> KDIEISASESKFILEALRQNYRLDGRSFDQFRDVEITFGKEFGDVSVKMGNTKVHCRISCQIAQPYEDRPFEGLFVISTEISPMAGSQFENGNITGEDEVLCSRIIEKSVRRSGALDVEGLCIVAGSKCWAVRADVHFLDCDGGFIDASCIAVMAGLMHFKKPDITVHGEQIIVHPVNEREPVP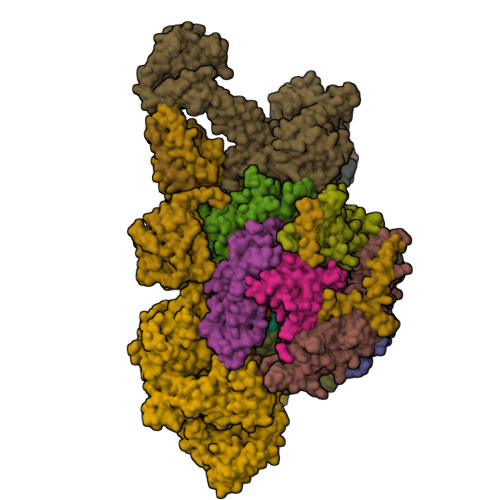LGILHIPICVTFSFFNPQDTEENIKGETNSEISIIDATLKEELLRDGVLTVTLNKNREVVQVSKAGGLPMDALTLMKCCHEAYSIIEKITDQILQLLKEDSEKRNKYAAMLTSENAREI;> GHMSRLEIYSPEGLRLDGRRWNELRRFESSINTHPHAADGSSYMEQGNNKIITLVKGPKEPRLKSQMDTSKALLNVSVNITKFSKFERSKSSHKNERRVLEIQTSLVRMFEKNVMLNIYPRTVIDIEIHVLEQDGGIMGSLINGITLALIDAGISMFDYISGISVGLYDTTPLLDTNSLEENAMSTVTLGVVGKSEKLSLLLVEDKIPLDRLENVLAIGIAGAHRVRDLMDEELRKHAQKRVSNASAR;> AESTTLETIEIHPITFPPEVLARISPELSLQRHLSLGIRPCLRKYEEFRDVAIENNTLSRYADAGNIDTKNNILGSNVLKSGKTIVITSITGGIIEETSASIKDLDDFGEEELFEVTKEEDIIANYASVYPVVEVERGRVGACTDEEMTISQKLHDSILHSRILPKKALKVKAGVRSANEDGTFSVLYPDELEDDTLNETNLKMKRKWSYVLYAKIVVLSRTGPVFDLCWNSLMYALQSVKLPRAFIDERASDLRMTIRTRGRSATIRETYEIICDQTKSVPLMINAKNIAFASNYGIVELDPECQLQNSDNSEEEEVDIDMDKLNTVLIADLDTEAEETSIHSTISILAAPSGNYKQLTLMGGGAKITPEMIKRSLLLSRVRADDLSTRFNI;> GHGNNKEPNTKNRLDSAEKKKKMSVQAEIGILDHVDGSSEFVSQDTKVICSVTGPIEPKARQELPTQLALEIIVRPAKGVATTREKVLEDKLRAVLTPLITRHCYPRQLCQITCQILESGEDEAEFSLRELSCCINAAFLALVDAGIALNSMCASIPIAIIKDTSDIIVDPTAEQLKISLSVHTLALEFVNGGKVVKNVLLLDSNGDFNEDQLFSLLELGEQKCQELVTNIRRIIQDNISPRLVV;> GHMSLSVAEKSYLYDSLASTPSIRPDGRLPHQFRPIEIFTDFLPSSNGSSRIIASDGSECIVSIKSKVVDHHVENELLQVDVDIAGQRDDALVVETITSLLNKVLKSGSGVDSSKLQLTKKYSFKIFVDVLVISSHSHPISLISFAIYSALNSTYLPKLISAFDDLEVEELPTFHDYDMVKLDINPPLVFILAVVGNNMLLDPAANESEVANNGLIISWSNGKITSPIRSVALNDSNVKSFKPHLLKQGLAMVEKYAPDVVRSLENL;> MNVQDRRRLLGPAAAKPMAFSNTTTHVPEKKSTDLTPKGNESEQELSLHTGFIENCNGSALVEARSLGHQTSLISAVYGPRSIRGSFTSQGTISIQLKNGLLEKYNTNELKEVSSFLMGIFNSVVNLSRYPKSGIDIFVYLTYDKDLTNNPQDDDSQSKMTSSQISSLIPHCITSITLALADAGIELVDMAGAGEANGTVVSFIKNGEEIVGFWKDDGDDEDLLECLDRCKEQYNRYRDLMISCLMNQET;> GHMSTFIFPGDSFPVDPTTPVKLGPGIYCDPNTQEIRPVNTGVLHVSAKGKSGVQTAYIDYSSKRYIPSVNDFVIGVIIGTFSDSYKVSLQNFSSSVSLSYMAFPNASKKNRPTLQVGDLVYARVCTAEKELEAEIECFDSTTGRDAGFGILEDGMIIDVNLNFARQLLFNNDFPLLKVLAAHTKFEVAIGLNGKIWVKCEELSNTLACYRTIMECCQKNDTAAFKDIAKRQFKEILTVKEE;> RSMSEVITITKRNGAFQNSSNLSYNNTGISDDENDEEDIYMHDVNSASKSESDSQIVTPGELVTDDPIWMRGHGTYFLDNMTYSSVAGTVSRVNRLLSVIPLKGRYAPETGDHVVGRIAEVGNKRWKVDIGGKQHAVLMLGSVNLPGGILRRKSESDELQMRSFLKEGDLLNAEVQSLFQDGSASLHTRSLKYGKLRNGMFCQVPSSLIVRAKNHTHNLPGNITVVLGVNGYIWLRKTSQMDLARDTPSANNSSSIKSTGPTGAVSLNPSITRLEEESSWQIYSDENDPSISNNIRQAICRYANVIKALAFCEIGITQQRIVSAYEASMVYSNVGELIEKNVMESIGSDILTAEKMRGNGN;> MKHHHHHHPMACNFQFPEIAYPGKLICPQYGTENKDGEDIIFNYVPGPGTKLIQYEHNGRTLEAITATLVGTVRCEEEKKTDQEEEREGTDQSTEEEKSVDASPNDVTRRTVKNILVSVLPGTEKGRKTNKYANNDFANNLPKEGDIVLTRVTRLSLQRANVEILAVEDKPSPIDSGIGSNGSGIVAAGGGSGAATFSVSQASSDLGETFRGIIRSQDVRSTDRDRVKVIECFKPGDIVRAQVLSLGDGTNYYLTTARNDLGVVFARAANGAGGLMYATDWQMMTSPVTGATEKRKCAKPF;> GAMSVPAIAPRRKRLADGLSVTQKVFVRSRNGGATKIVREHYLRSDIPCLSRSCTKCPQIVVPDAQNELPKFILSDSPLELSAPIGKHYVVLDTNVVLQAIDLLENPNCFFDVIVPQIVLDEVRNKSYPVYTRLRTLCRDSDDHKRFIVFHNEFSEHTFVERLPNETINDRNNRAIRKTCQWYSEHLKPYDINVVLVTNDRLNREAATKEVESNIITKSLVQYIELLPNADDIRDSIPQMDSFDKDLERDTFSDFTFPEYYSTARVMGGLKNGVLYQGNIQISEYNFLEGSVSLPRFSKPVLIVGQKNLNRAFNGDQVIVELLPQSEWKAPSSIVLDSEHFDVNDNPDIEAGDDDDNNESSSNTTVISDKQRRLLAKDAMIAQRSKKIQPTAKVVYIQRRSWRQYVGQLAPSSVDPQSSSTQNVFVILMDKCLPKVRIRTRRAAELLDKRIVISIDSWPTTHKYPLGHFVRDLGTIESAQAETEALLLEHDVEYRPFSKKVLECLPAEGHDWKAPTKLDDPEAVSKDPLLTKRKDLRDKLICSIDPPGCVDINDALHAKKLPNGNWEVGVHIADVTHFVKPGTALDAEGAARGTSVYLVDKRIDMLPMLLGTDLCSLKPYVDRFAFSVIWELDDSANIVNVNFMKSVIRSREAFSYEQAQLRIDDKTQNDELTMGMRALLKLSVKLKQKRLEAGALNLASPEVKVHMDSETSDPNEVEIKKLLATNSLVEEFMLLANISVARKIYDAFPQTAMLRRHAAPPSTNFEILNEMLNTRKNMSISLESSKALADSLDRCVDPEDPYFNTLVRIMSTRCMMAAQYFYSGAYSYPDFRHYGLAVDIYTHFTSPIRRYCDVVAHRQLAGAIGYEPLSLTHRDKNKMDMICRNINRKHRNAQFAGRASIEYYVGQVMRNNESTETGYVIKVFNNGIVVLVPKFGVEGLIRLDNLTEDPNSAAFDEVEYKLTFVPTNSDKPRDVYVFDKVEVQVRSVMDPITSKRKAELLLK;> MTSENPDVLLSRVINVVRAASSLASQDVDFYKNLDRGFSKDLKSKADKLADMANEIILSIDEHHESFELKEEDISDLWNNFGNIMDNLLEMSDHSLDKLNCAINSKSRGSDLQYLGEFSGKNFSPTKRVEKPQLKFKSPIDNSESHPFIPLLKEKPNALKPLSESLRLVDDDENNPSHYPHPYEYEIDHQEYSPEILQIREEIPSKSWDDSVPIWVDTSTELESMLEDLKNTKEIAVDLEHHDYRSYYGIVCLMQISTRERDYLVDTLKLRENLHILNEVFTNPSIVKVFHGAFMNIIWLQRDLGLYVVGLFDTYHASKAIGLPRHSLAYLLENFANFKTSKKYQLADWRIRPLSKPMTAYARADTHFLLNIYDQLRNKLIESNKLAGVLYESRNVAKRRFEYSKYRPLTPSSEVYSPIEKESPWKILMYQYNIPPEREVLVRELYQWRDLIARRDDESPRFVMPNQLLAALVAYTPTDVIGVVSLTNGVTEHVRQNAKLLANLIRDALRNIKNTNEEATPIPSSETKADGILLETISVPQIRDVMERFSVLCNSNISKSRAKPVTNSSILLGKILPREEHDIAYSKDGLPNKVKTEDIRIRAQNFKSALANLEDIIFEIEKPLVVPVKLEEIKTVDPASAPNHSPEIDNLDDLVVLKKKNIQKKQPAKEKGVTEKDAVDYSKIPNILSNKPGQNNRQQKKRRFDPSSSDSNGPRAAKKRRPAAKGKNLSFKR;> MEDIEKIKPYVRSFSKALDELKPEIEKLTSKSLDEQLLLLSDERAKLELINRYAYVLSSLMFANMKVLGVKDMSPILGELKRVKSYMDKAKQYDNRITKSNEKSQAEQEKAKNIISNVLDGNKNQFEPSISRSNFQGKHTKFENDELAESTTTKIIDSTDHIRKASSKKSKRLDKVGKKKGGKK;> MDSTDLFDVFEETPVELPTDSNGEKNADTNVGDTPDHTQDKKHGLEEEKEEHEENNSENKKIKSNKSKTEDKNKKVVVPMLADSFEQEASREVDASKGLTNSETLQVEQDGKVRLSHQVRHQVALPPNYDYTPIAEHKRVNEARTYPFTLDPFQDTAISCIDRGESVLVSAHTSAGKTVVAEYAIAQSLKNKQRVIYTSPIKALSNQKYRELLAEFGDVGLMTGDITINPDAGCLVMTTEILRSMLYRGSEVMREVAWVIFDEVHYMRDKERGVVWEETIILLPDKVRYVFLSATIPNAMEFAEWICKIHSQPCHIVYTNFRPTPLQHYLFPAHGDGIYLVVDEKSTFREENFQKAMASISNQIGDDPNSTDSRGKKGQTYKGGSAKGDAKGDIYKIVKMIWKKKYNPVIVFSFSKRDCEELALKMSKLDFNSDDEKEALTKIFNNAIALLPETDRELPQIKHILPLLRRGIGIHHSGLLPILKEVIEILFQEGFLKVLFATETFSIGLNMPAKTVVFTSVRKWDGQQFRWVSGGEYIQMSGRAGRRGLDDRGIVIMMIDEKMEPQVAKGMVKGQADRLDSAFHLGYNMILNLMRVEGISPEFMLEHSFFQFQNVISVPVMEKKLAELKKDFDGIEVEDEENVKEYHEIEQAIKGYREDVRQVVTHPANALSFLQPGRLVEISVNGKDNYGWGAVVDFAKRINKRNPSAVYTDHESYIVNVVVNTMYIDSPVNLLKPFNPTLPEGIRPAEEGEKSICAVIPITLDSIKSIGNLRLYMPKDIRASGQKETVGKSLREVNRRFPDGIPVLDPVKNMKIEDEDFLKLMKKIDVLNTKLSSNPLTNSMRLEELYGKYSRKHDLHEDMKQLKRKISESQAVIQLDDLRRRKRVLRRLGFCTPNDIIELKGRVACEISSGDELLLTELIFNGNFNELKPEQAAALLSCFAFQERCKEAPRLKPELAEPLKAMREIAAKIAKIMKDSKIEVVEKDYVESFRHELMEVVYEWCRGATFTQICKMTDVYEGSLIRMFKRLEELVKELVDVANTIGNSSLKEKMEAVLKLIHRDIVSAGSLYL3-[[6-~{tert}-butyl-2-[3-(dimethylamino)propyl-methyl-amino]thieno[3,2-d]pyrimidin-4-yl]-methyl-amino]propanenitrile | C20 H32 N6 S | 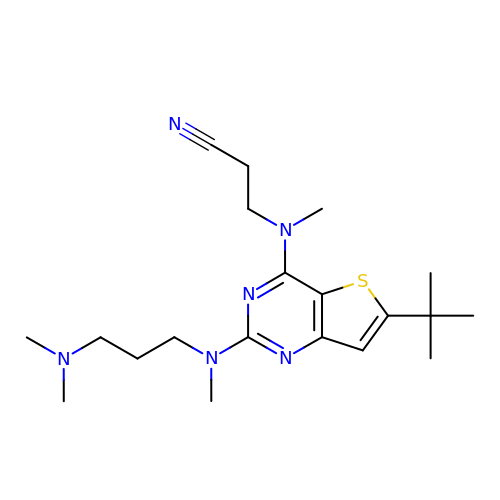IEVFUBDHAUXBHH-UHFFFAOYSA-N> MGIVGVGIDLVSIPDFAEQVDQPGTVFMETFTPGERRDASDKSSSAARHLAARWAAKEAVIKAW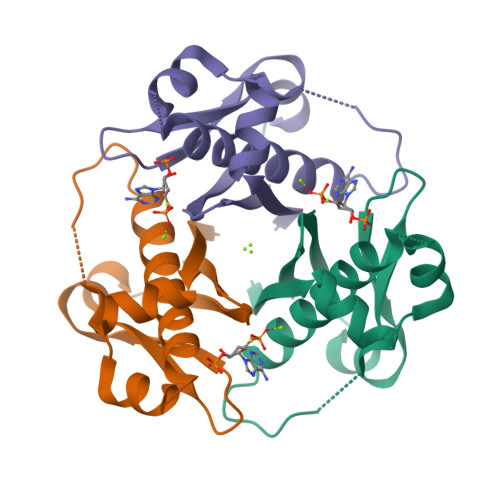SGSRFAQRPMLPEDIHRDIEVVTDMWGRPRVRLTGAIAEYLADVTIHVSLTHEGDTAAAVAILEAP>[2x]MENISPGQIIDEPIRPVNIPRKEKDFQGMLEYKKEDEQKLVKNLILELKPRGVAVNLIPGLPAYILFMCVRHADYLNDDQKVRSLLTSTINSIKKVLKKRGDDFETVSFWLSNTCRFLHCLKQYSGEEGFMKHNTSRQNEHCLTNFDLA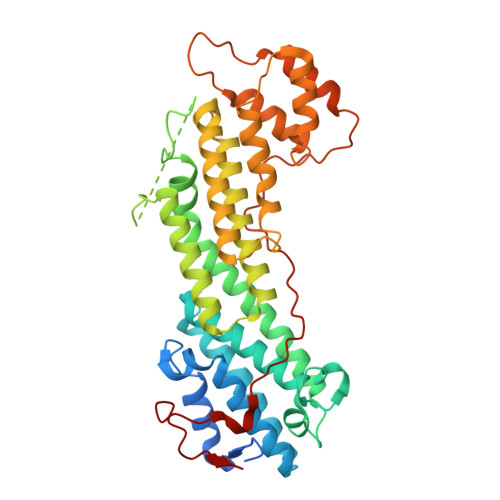EYRQVLSDLAIQIYQQLVRVLENILQPMIVSGMLEHETIQGVSGVKPTGLRKRTSSIADEGTYTLDSILRQLNSFHSVMCQHGMDPELIKQVVKQMFYIIGAITLNNLLLRKDMCSWSKGMQIRYNVSQLEEWLRDKNLMNSGAKETLEPLIQAAQLLQVKKKTDDDAEAICSMCNALTTAQIVKVLNLYTPVNEFEERVSVSFIRTIQMRLRDRKDSPQLLMDAKHIFPVTFPFNPSSLALETIQIPASLGLGFISRV> 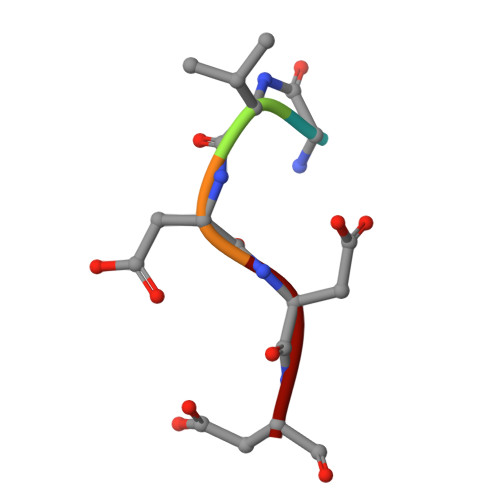GVDDD>DEGKLTGGQSPATSTQNNESAEADMQQQQSKEMSQEMETLMESIKKALEREIEQGAIEVENLGQQIVIRMREKGAFPEGSAFLQPKFRPLVRQIAELVKDVPGIVRVSGHTDNRPLDSELYRSNWDLSSQRAVSVAQEMEKVRGFSHQRLRVRGMADTEPLLPNDSDDNRALNRRVEISIMQGEPLYSEEVPVIQHH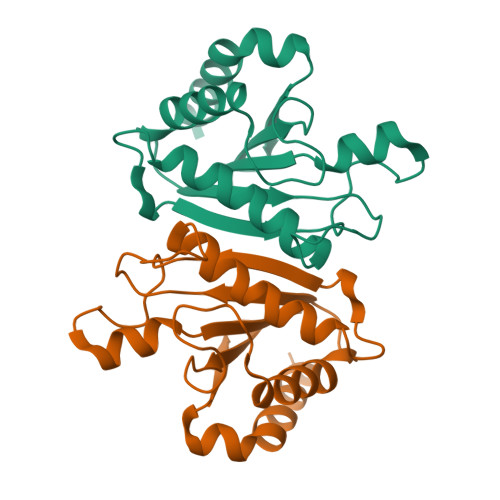HHHH[2x]TATA box-binding protein (TBP) is a key protein that facilitates transcription of ribosomal RNAs (rRNAs), messenger RNAs (mRNAs), and transfer RNAs (tRNAs) by the three eukaryotic RNA polymerases: Pol I, Pol II and Pol III, respectively. The concave hydrophobic surface of TBP interacts with the minor groove of the DNA, whereas the highly charged convex surface mediates binding with diverse transcription regulators. A group of nuclear transport receptors, collectively termed karyopherin-β (Kap-β) in yeast, facilitates active nucleo-cytoplasmic transport. In previous studies we showed that Kap114p, a Kap-β that mediates nuclear import of yeast TBP (yTBP), modulates yTBP-dependent transcription.

Ultimately, a cryo-EM structure of the Kap114•yTBPC complex, representing a ~130 kDa heterodimeric protein complex, was determined to an average resolution of 4.03 Å using 212,899 particles. In the Kap114•yTBPC complex, Kap114p is arranged into a right-handed superhelix and forms a 1:1 stoichiometric complex with yTBPC. Notably, Kap114p mainly wraps around the pseudosymmetric N-terminal lobe of yTBPC, primarily via three binding patches (the B α-helix and loop of HEAT8, the B α-helix of HEAT13, and the α-helix of the HEAT19 loop; highlighted by light blue, light green and light orange in Fig. 1c–e). A short α-helix in the Kap114p HEAT19 loop binds to the hydrophobic concave surface of yTBPC in a similar way to the TAF N-terminal domain (TAND) of TAF1 and a latch region of Mot121,24. Residue Y939 of Kap114p interacts with yTBPC Q158, just as F23 of TAF1-TAND1 binds to Q158 of yTBP and F123 of Mot1 binds to Q116 of EcTBP. Residues Y933 of Kap114p and F99 of yTBPC facilitate hydrophobic interactions, comparable to those of Mot1 F129 to EcTBP F57/F74 and TAF1-TAND1 Y19 to yTBP F99/F116. Among these five residues, R90 and N91, located near the α-helix 1 of yTBPC, are bound by the HEAT8 loop of Kap114p and exhibit close contacts with the HEAT8 loop via residues S369 and Y370. The other three signature residues—R137, R141 and K145—are located at α-helix 2 of yTBPC and interact with the HEAT8 loop and HEAT13B. In particular, the double mutant combining Y370A on Kap114p and N91A on yTBPC resulted in a Kd value of ~1.5 μM for the complex, i.e., more than a thousand-fold weaker than wild type. Hence, Kap114p binding does not induce substantial conformational changes in yTBPC, consistent with our understanding of how other TBP-associated factors promote TBP remodeling as a consequence of binding without changing the TBP structure.

> MDINELIIGAQSADKHTREVAETQLLQWCDSDASQVFKALANVALQHEASLESRQFALLSLRKLITMYWSPGFESYRSTSNVEIDVKDFIREVLLKLCLNDNENTKIKNGASYCIVQISAVDFPDQWPQLLTVIYDAISHQHSLNAMSLLNEIYDDVVSEEMFFEGGIGLATMEIVFKVLNTETSTLIAKIAALKLLKACLLQMSSHNEYDEASRKSFVSQCLATSLQILGQLLTLNFGNVDVISQLKFKSIIYENLVFIKNDFSRKHFSSELQKQFKIMAIQDLENVTHINANVETTESEPLLETVHDCSIYIVEFLTSVCTLQFSVEEMNKIITSLTILCQLSSETREIWTSDFNTFVSKETGLAASYNVRDQANEFFTSLPNPQLSLIFKVVSNDIEHSTCNYSTLESLLYLLQCILLNDDEITGENIDQSLQILIKTLENILVSQEIPELILARAILTIPRVLDKFIDALPDIKPLTSAFLAKSLNLALKSDKELIKSATLIAFTYYCYFAELDSVLGPEVCSETQEKVIRIINQVSSDAEEDTNGALMEVLSQVISYNPKEPHSRKEILQAEFHLVFTISSEDPANVQVVVQSQECLEKLLDNINMDNYKNYIELCLPSFINVLDSNNANNYRYSPLLSLVLEFITVFLKKKPNDGFLPDEINQYLFEPLAKVLAFSTEDETLQLATEAFSYLIFNTDTRAMEPRLMDIMKVLERLLSLEVSDSAAMNVGPLVVAIFTRFSKEIQPLIGRILEAVVVRLIKTQNISTEQNLLSVLCFLTCNDPKQTVDFLSSFQIDNTDALTLVMRKWIEAFEVIRGEKRIKENIVALSNLFFLNDKRLQKVVVNGNLIPYEGDLIITRSMAKKMPDRYVQVPLYTKIIKLFVSELSFQSKQPNPEQLITSDIKQEVVNANKDDDNDDWEDVDDVLDYDKLKEYIDDDVDEEADDDSDDITGLMDVKESVVQLLVRFFKEVASKDVSGFHCIYETLSDSERKVLSEALL;> SGIVPTLQNIVATVTLGCRLDLKTVALHARNAEYNPKRFAAVIMRIREPKTTALIFASGKMVVTGAKSEDDSKLASRKYARIIQKIGFAAKFTDFKIQNIVGSCDVKFPIRLEGLAFSHGTFSSYEPELFPGLIYRMVKPKIVLLIFVSGKIVLTGAKQREEIYQAFEAIYPVLSEFRKM> XPLAS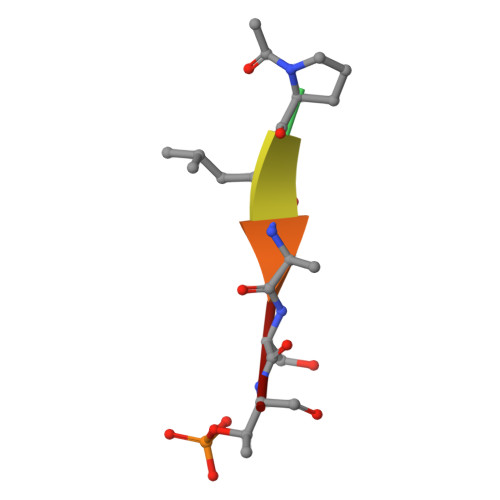T> MTARNPLEAQAWALLEAVYDPELGLDVVNLGLIYDLVVEPPRAYVRMTLTTPGCPLHDSLGEAVRQALSRLPGVEEVEVEV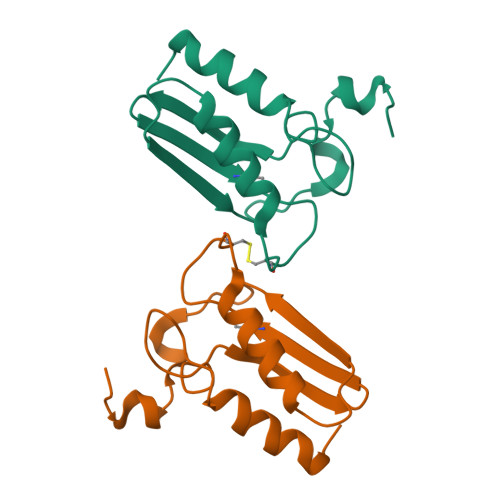TFEPPWTLARLSEKARRLLGWG N-(1-benzofuran-2-ylmethyl)-N'-(1,2,3,4-tetrahydroacridin-9-yl)heptane-1,7-diamine | C29 H35 N3 O | 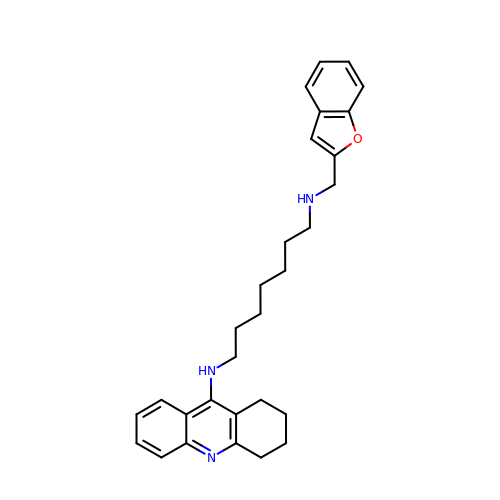LJASCSHXLYLOCF-UHFFFAOYSA-N> AFGITTSSSAYVIDTNAPNQLKFTVSRSSCDITSIIHYGTELQYSSQGSHIGSGLGSATVTATQSGDYIKVTCVTDTLTQYMVVHNGDPIIHMATYITAEPSIGELRFIARLNSDLLPNEEPFGDVSTTADGTAIEGSDVFLVGSETRSKFY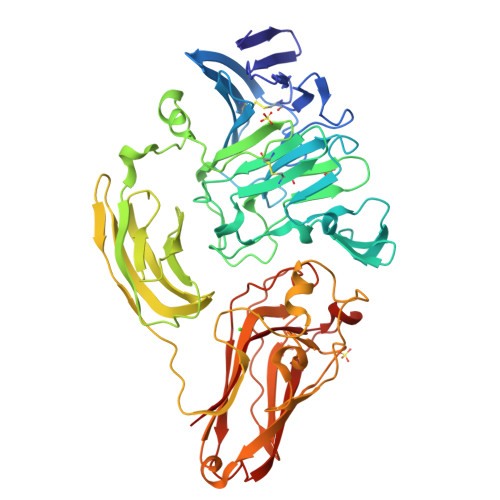SSERFIDDQRHCIAGDAHRVCMILNQYESSSGGPFHRDINSNNGGSYNALYWYMNSGAVQTESYRMGLHGPYSMYFSRSGTPSTSIDTSFFADLDIKGYVAASGRGKVAGTASGADSSMDWVVHWYNDAAQYWTYTSSSGSFTSPAMKPGTYTMVYYQGEYAVATSSVTVSAGSTTTKNISGSVKTGTTIFKIGEWDGQPTGFRNAANQLRMHPSDSRMSSWGPLTYTVGSSALTDFPMAVFKSVNNPVTIKFTATSAQTGAATLRIGTTLSFAGGRPQATINSYTGSAPAAPTNLDSRGVTRGAYRGLGEVYDVSIPSGTIVAGTNTITINVISGSSGDTYLSPNFIFDCVELFQ>[6x]MTSAEMTSPNNNS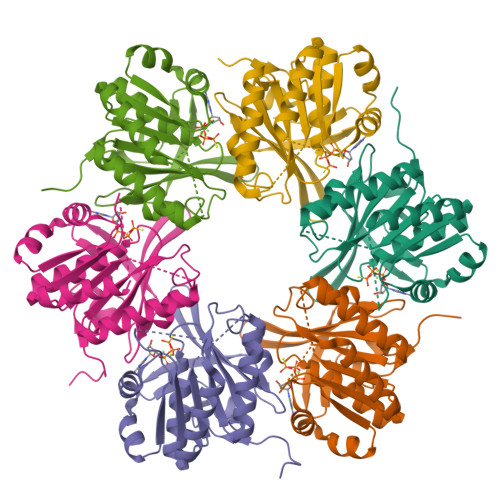EHQAIAKMRTMIEGFDDISHGGLPIGRSTLVSGTSGTGKTLFSIQFLYNGIIEFDEPGVFVTFEETPQDIIKNARSFGWDLAKLVDEGKLFILDASPDPEGQEVVGGFDLSALIERINYAIQKYRARRVSIDSVTSVFQQYDACSVVRRELFRLVARLKQIGATTVMTTERIEEYGPIARYGVEEFVSDNVVILRNVLEGERRRRTLEILKLRGTSHMKGEYPFTITDHGINIFPLGAMR>ATKVAVAGASGYAGGEILRLLLGHPAYADGRLRIGALTAATSAGSTLGEHHPHLTPLAHRVVEPTEAAVLGGHDAVFLALPHGHSAVLAQQLSPETLIIDCGADFRLTDAAVWERFYGSSHAGSWPYGLPELPGARDQLRGTRRIAVPGCYPTAALLALFPALAADLIEPAVTVVAVSGTSGAGRAATTDLLGAEVIGSARAYNI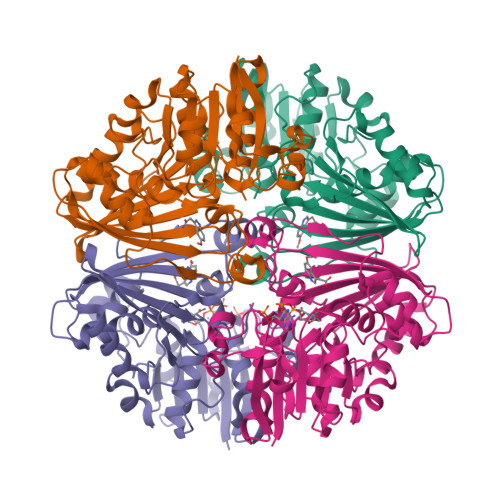AGVHRHTPEIAQGLRAVTDRDVSVSFTPVLIPASRGILATCTARTRSPLSQLRAAYEKAYHAEPFIYLMPEGQLPRTGAVIGSNAAHIAVAVDEDAQTFVAIAAIDNLVKGTAGAAVQSMNLALGWPETDGLSVVGVAP[8x]>[2x]MRGSAFNGKWETESQEGYEPFCKLIGIPDDVIAKGRDFKLVTEIVQNGDDFTWTQYYPNNHVVTNKFIVGKESDMETVGGKKFKGIVSMEGGK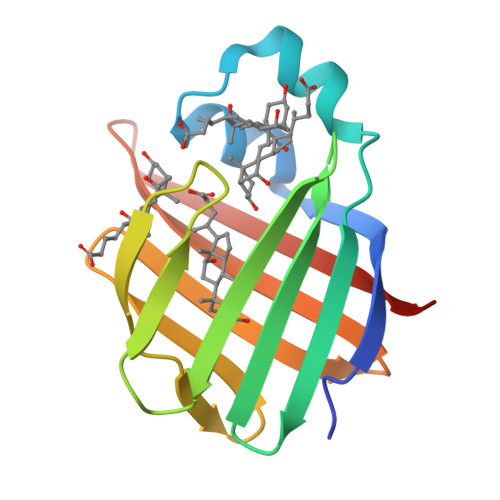LTISFPKYQQTTEISGGKLVETSTASGAQGTAVLVRTSKKVLVPR>GMQENTRLRIAIQKSGRLSKESIELLSECGVKMHIHEQSLIAFSTNLPIDILRVRDDDIPGLIFDGVVDLGIIGENVLEENELERQSLGENPSYKLLKKLDFGYCRLSLALPQENKFQNLKDFEGLRIATSYPQLLKRFMKENGINYKNCTLTGSVEVAPRANLADAICDLVSSGATLQANNLKEVKVIYESRACLIQKENALSKEKQALVDKIMLRVAGVMQARESKYIMLHAPKEKLDKIQALLPGVERPTILPLAHDEKNVALHMVS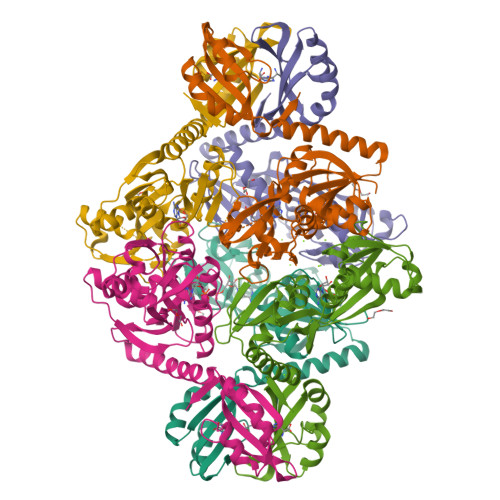KENLFWETMEALKEEGASSILVLPIEKMLK[6x]(3~{S},3'~{R},3'~{a}~{S},6'~{a}~{R})-6-chloranyl-3'-(3-chloranyl-2-fluoranyl-phenyl)-1'-(cyclopropylmethyl)spiro[1~{H}-indole-3,2'-3~{a},6~{a}-dihydro-3~{H}-pyrrolo[3,4-b]pyrrole]-2,4'-dione 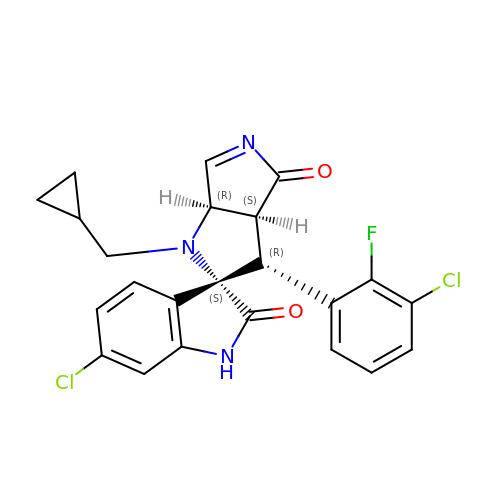| C23 H18 Cl2 F N3 O2 | ZWMAKFAKGSTVDL-QPXQOZNCSA-N>[2x]GMTAPTLSR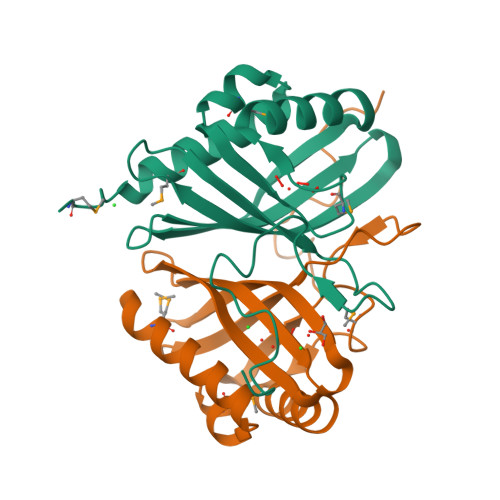AAMEKVIRTYYDGCNEADEAKMIACFVPEAVHYFPAGMYGGAFRGAAQIAHRWRTAVETLGSYWTIDALVIDAETAEAAIEWTHFKTNQDKVLRGAECVEFDRASGLIREIRAFYASPQAEGIARLELGDFDYAGRGYRVTSPRKPA> MSISISYSTTYSGWTVADYLADWSAYFGDVNHRPGQVVDGSNTGGFNPGPFDGSQYALKSTASDAAFIAGGDLHYTLFSNPSHTLWGKLDSIALGDTLTGGASSGGYALDSQEV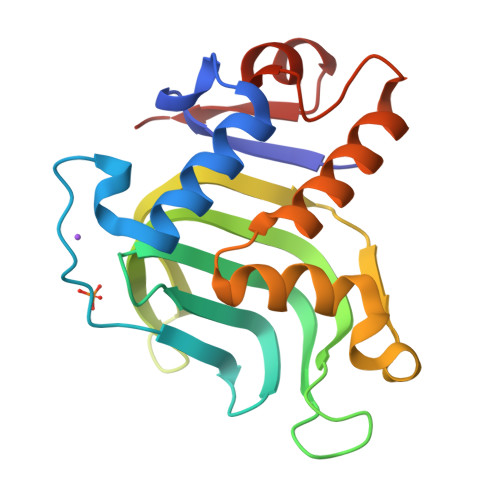SFSNLGLDSPIAQGRDGTVHKVVYGLMSGDSSALQGQIDALLKAVDPSLSINSTFDQLAAAGVAHATPAA The RecA family of DNA strand exchange proteins exists in all three kingdoms of life. Members of the RecA protein family include prokaryotic RecA, archaeal RadA and Rad51, and eukaryotic Rad51 and Dmc1. These proteins play a central role in homologous recombination, an error-free DNA repair mechanism [for reviews see 1]. Members of RecA family all contain a central ATPase domain that is preceded by a short β-stranded polymerization motif (PM).

In this study, we present the crystal structure of SsoRadA 31 overwound right-handed filament at 1.93Å resolution. In the final 1.93Å resolution crystal structure, SsoRadA protomers are packed into three extended helical filaments in a 98Å pitch helix with three protomers per turn. In contrast, chain A does not contain a visible NTD and has an average B-value of 48.2 Å2. As in other filamentous structures of archaeal and eukaryotic RecA family proteins, a conserved amino acid residue (Phe73) in the PM is responsible for the assembly of the 31 overwound right-handed SsoRadA filament. Phe73 is docked into a hydrophobic pocket (which includes Val145, Tyr177, Ile190, Asp193, Leu194, and Leu197) of the neighboring protomer. Intriguingly, the overwound right-handed SsoRadA filament contains ordered polypeptide backbones and side-chains in two important structural regions, L1 motif (amino acid residues 219–226) and NTD (amino acid residues 14–69), compared to those found in the previous lower resolution P3121 form. A surface charge potential analysis of the L1 motif reveals a linear basic patch on one face of the motif. This linear basic patch of SsoRadA L1 motif consists of three arginine residues (i.e., Arg217, Arg223, and Arg229), with their positively charged side chains directed upward. Surface potential analysis of the entire (HhH)2 domain of SsoRadA protein revealed a 92° arched basic patch along the border of the second HhH motif. Two lysine residues (i.e., Lys27 and Lys60) are located at each end of this arched basic patch. A closer look at this structure revealed that the linear basic patch of the L1 motif faces the arched basic patch of the (HhH)2 domains at a distance of ∼25 Å. Together, they constitute an outwardly open palm structure with its inner pocket containing five positively charged amino acid residues, i.e., R217, R223, R229 of the L1 motif and K27, K60 of the NTD.

>[3x]MSNEVEQKKNIKTINDLPGISQTVINKLIEAGYSSLETLAVASPQDLSVAAGIPLSTAQKIIKEARDALDIRFKTALEVKKERMNVKKISTGSQALDGLLAGGIETRTMTEFFGEFGSGKTQLCHQLSVNVQLPPEKGGLSGKAVYIDTEGTFRWERIENMAKALGLDIDNVMNNIYYIRAINTDHQIAIVDDLQELVSKDPSIKLIVVDSVTSHFRAEYPGRENLAVRQQKLNKHLHQLTRLAEVYDIAVIITNQVMARPDMFYGDPTVAVGGHTLYHVPGIRIQLKKSRGNRRIARVVDAPHLPEGEVVFALTEEGIRDAEE>MIISEFDRNNPVLKDQLSDLLRLTWPEEYGDSSAEEVEEMMNPERIAVAAVDQDELVGFIGAIPQYGITGWELHPLVVESSRRKNQIGTRLVNYLEKEVASRGGITIYLGTDDLDHGTTLSQTDLYEHTFDKVASIQNLREHPYEFYEKLGYKIVGVLPNANGWDK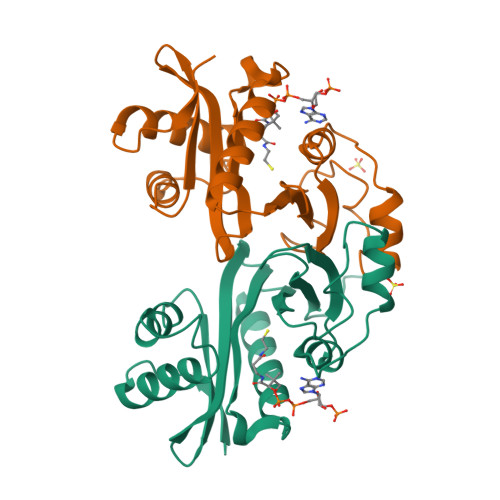PDIWMAKTIIPRPDSQ[2x]>GMPTETFF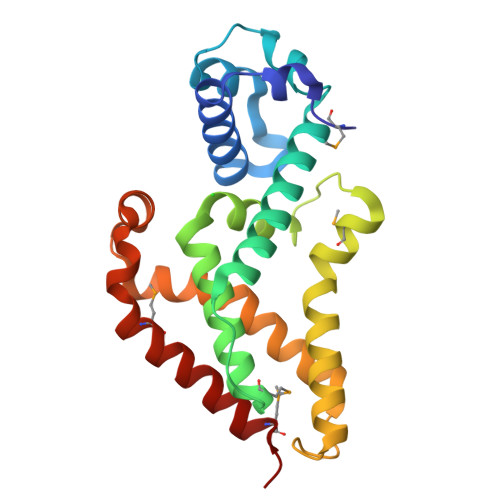NLPEEKRSRLIDVLLDEFAQNDYDSVSINRITERAGIAKGSFYQYFADKKDCYLYLIQLGIEQKTAFLRQTPPASTTDMFAYLRWLLDVGIQFQFHNPRLAQIAYKALYDDVPLPAETMQVIRHGSFAYFKQLVEQGIADGSLVPDLDADTAAFVLNVVFTELGNHLIERFAVNPAELLREGGIVLLQPAMRRVIEQVIDILERGMRRR[5x]> MATATEQWVLVEMVQALYEAPAYHLILEGILILWIIRLLFSKTYKLQERSDLTVKEKEELIEEWQPEPLVPPVPKDHPALNYNIVSGPPSHKTVVNGKECINFASFNFLGLLDNPRVKAAALASLKKYGVGTCGPRGFYGTFDVHLDLEDRLAKFMKTEEAIIYSYGFATIASAIPAYSKRGDIVFVDRAACFAIQKGLQASRSDIKLFKHNDMADLERLLKEQEIEDQKNPRKARVTRRFIVVEGLYMNTGTICPLPELVKLKYKYKARIFLEESLSFGVLGEHGRGVTEHYGINIDDIDLISANMENALASIGGFCCGRSFVIDHQRLSGQGYCFSASLPPLLAAAAIEALNIMEENPGIFAVLKEKCGQIHKALQGISGLKVVGESLSPAFHLQLEESTGSREQDVRLLQEIVDQCMNRSIALTQARYLEKEEKCLPPPSIRVVVTVEQTEEELERAASTIKEVAQAVLL;> MRPEPGGCCCRRTVRANGCVANGEVRNGYVRSSAAAAAAAAAGQIHHVTQNGGLYKRPFNEAFEETPMLVAVLTYVGYGVLTLFGYLRDFLRYWRIEKCHHATEREEQ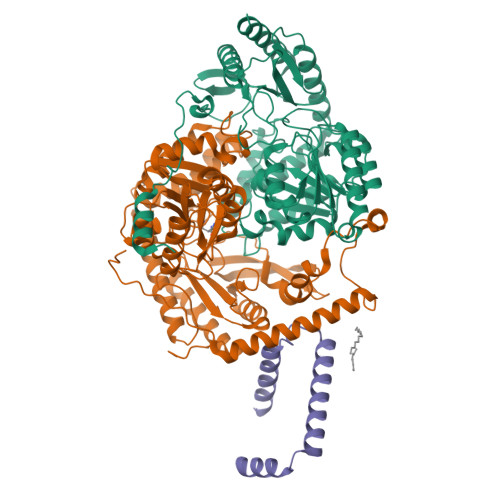KDFVSLYQDFENFYTRNLYMRIRDNWNRPICSVPGARVDIMERQSHDYNWSFKYTGNIIKGVINMGSYNYLGFARNTGSCQEAAAKVLEEYGAGVCSTRQEIGNLDKHEELEELVARFLGVEAAMAYGMGFATNSMNIPALVGKGCLILSDELNHASLVLGARLSGATIRIFKHNNMQSLEKLLKDAIVYGQPRTRRPWKKILILVEGIYSMEGSIVRLPEVIALKKKYKAYLYLDEAHSIGALGPTGRGVVEYFGLDPEDVDVMMGTFTKSFGASGGYIGGKKELIDYLRTHSHSAVYATSLSPPVVEQIITSMKCIMGQDGTSLGKECVQQLAENTRYFRRRLKEMGFIIYGNEDSPVVPLMLYMPAKIGAFGREMLKRNIGVVVVGFPATPIIESRARFCLSAAHTKEILDTALKEIDEVGDLLQLKYSRHRLVPLLDRPFDETTYEETED;> MAGMALARAWKQMSWFYYQYLLVTALYMLEPWERTVFNSMLVSIVGMALYTGYVFMPQHIMAILHYFEIVQ3-[1-(4-cyanophenyl)piperidin-4-yl]-~{N}-[(4-piperidin-1-ylphenyl)methyl]propanamide | C27 H34 N4 O | 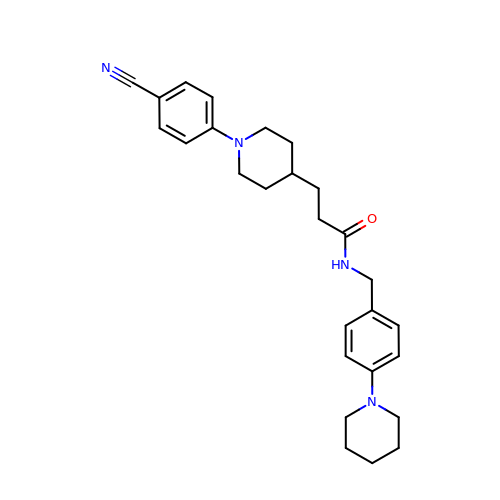JAVRLGIYSMGJKK-UHFFFAOYSA-N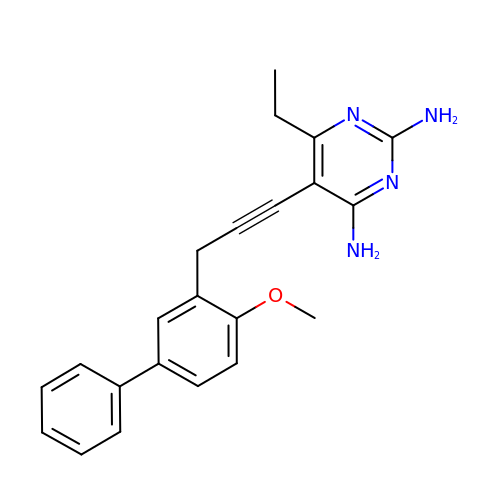6-ethyl-5-[3-(4-methoxybiphenyl-3-yl)prop-1-yn-1-yl]pyrimidine-2,4-diamine | C22 H22 N4 O | LBQMRSNKEUNXMT-UHFFFAOYSA-N> SVAILQKRDHEGFGFVLRGAKAETPIEEFTPTPAFPALQYLESVDVEGVAWKAGL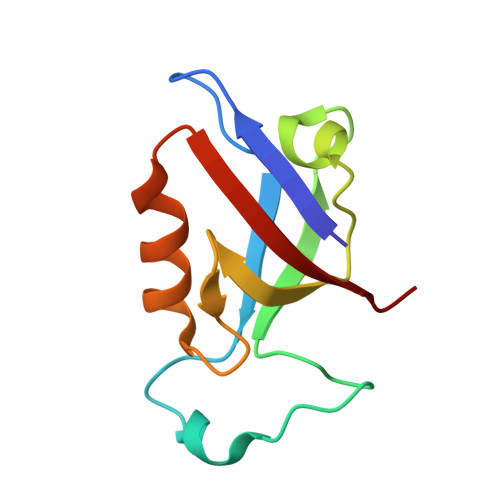RTGDFLIEVNGVNVVKVGHKQVVGLIRQGGNRLVMKVVSVT> MASEFKKKLFWRAVVAEFLAMILFIFISIGSALGFHYPIKSNQTTGAVQDNVKVSLAFGLSIATLAQSVGHISGAHLNPAVTLGLLLSCQISVLRAIMYIIAQCVGAIV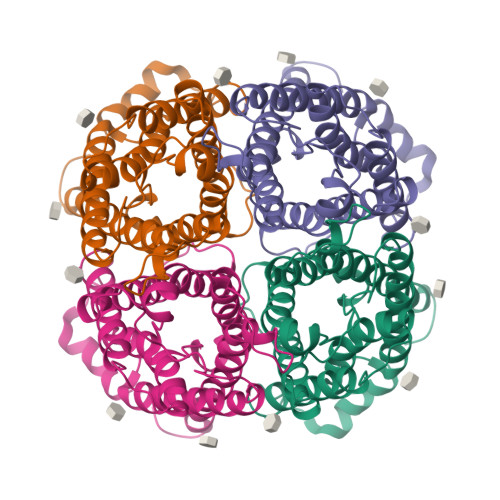ATAILSGITSSLPDNSLGLNALAPGVNSGQGLGIEIIGTLQLVLCVLATTDRRRRDLGGSGPLAIGFSVALGHLLAIDYTGCGINPARSFGSSVITHNFQDHWIFWVGPFIGAALAVLIYDFILAPRSSDLTDRVKVWTSGQVEEYDLDADDINSRVEMKPK5-[(4-methylbenzyl)oxy]quinazoline-2,4-diamine | C16 H16 N4 O | 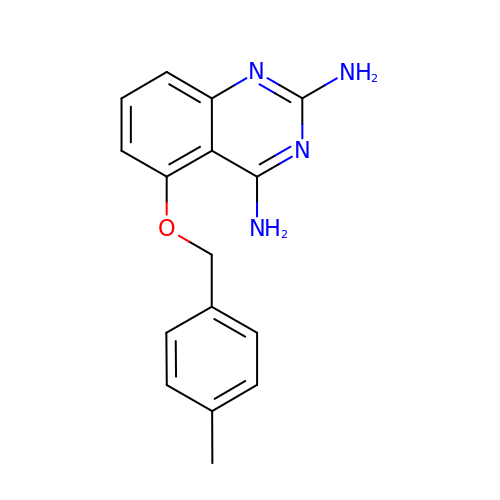XITJNLVILSJJHU-UHFFFAOYSA-N>[7x]MAIAQLATEYVFSDFLLKEPTEPKFKGLRLELAVDKMVTCIAVGLPLLLISLAFAQEISIGTQISCFSPSSFSWRQAAFVDSYCWAAVQQKNSLQSESGNLPLWLHKFFPYILLLFAILLYLPPLFWRFAAAPHICSDLKFIMEELDKVYNRAIKAAKSARDLDMRDGACSVPGVTENLGQSLWEVSESHFKYPIVEQYLKTKKNSNNLIIKYISCRLLTLIIILLAC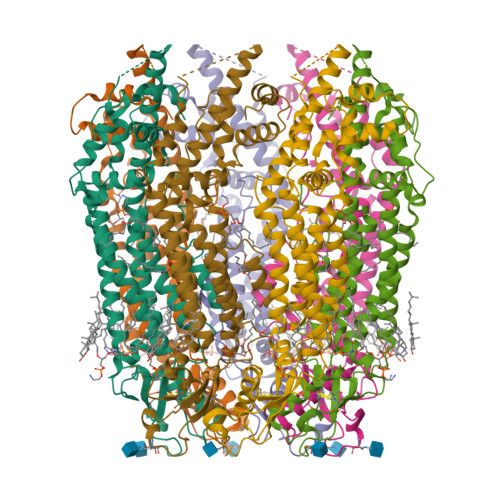IYLGYYFSLSSLSDEFVCSIKSGILRNDSTVPDQFQCKLIAVGIFQLLSVINLVVYVLLAPVVVYTLFVPFRQKTDVLKVYEILPTFDVLHFKSEGYNDLSLYNLFLEENISEVKSYKCLKVLENIKSSGQGIDPMLLLTNLGMI>[4x]MDYRTVFRLDGACAAVTGAGSGIGLEICRAFAASGARLILIDREAAALDRAAQELGAAVAARIVADVTDAEAMTAAAAEAEAVAPVSILVNSAGIARLH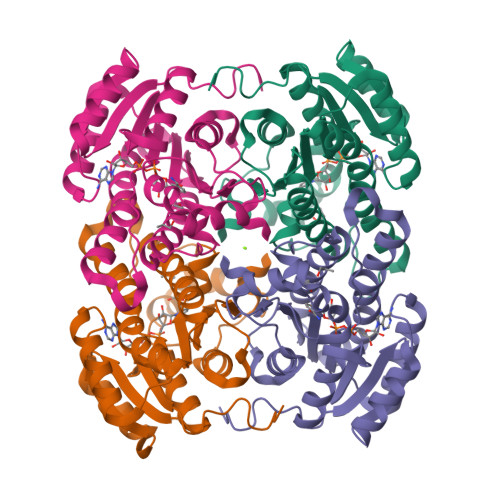DALETDDATWRQVMAVNVDGMFWASRAFGRAMVARGAGAIVNLGSMSGTIVNRPQFASSYMASKGAVHQLTRALAAEWAGRGVRVNALAPGYVATEMTLKMRERPELFETWLDMTPMGRCGEPSEIAAAALFLASPAASYVTGAILAVDGGYTVW>[4x]MIVVSGSQSQNLAFKVAKLLNTKLTRVEYKRFPDNEIYVRIVDEINDDEAVIINTQKNQNDAIVETILLCDALRDE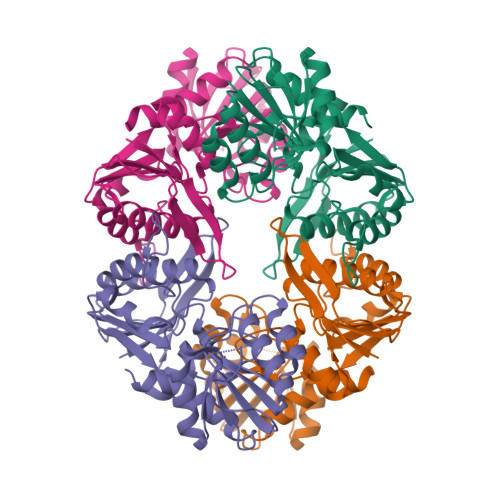GVKKITLVAPYLAYARQDKKFNPGEAISIRALAKIYSNIVDKLITINPHETHIKDFFTIPFIYGDAVPKLAEYVKDKLNDPIVLAPDKGALEFAKTASKILNAEYDYLEKTRLSPTEIQIAPKTLDAKDRDVFIVDDIISTGGTMATAVKLLKEQGAKKIIAACVHPVLIGDALNKLYSAGVEEVVGTDTYLSEVSKVSVAEVIVDLL>GUGTACA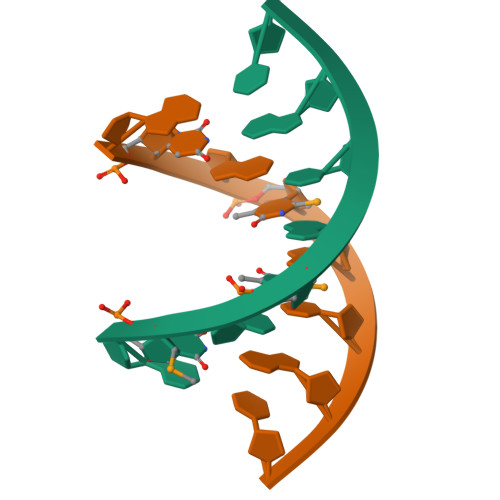C[2x]> QKVTFPKMKI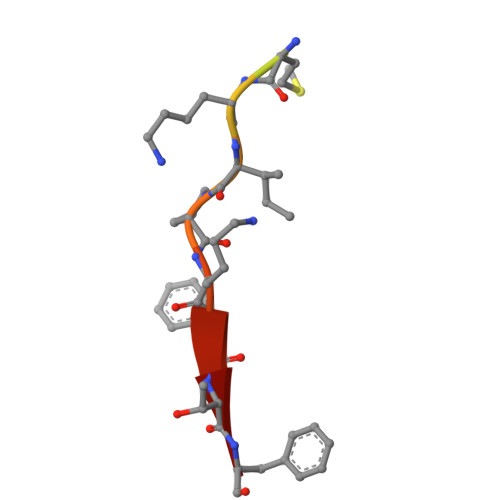PKFTF> LDFQALEETTEYDGGYTRDSVLIREFWEIVHSFTDEQKRLFLQFTTGTDRAPVGGLGKLKMIIAKNGPDTERLPTSHTCFNVLLLPEYSSKEKLKERLLKAITYA

The HECT‐type ubiquitin ligase E6AP (UBE3A) is critically involved in several neurodevelopmental disorders and human papilloma virus‐induced cervical tumorigenesis; the structural mechanisms underlying the activity of this crucial ligase, however, are incompletely understood. E3s of the HECT (homologous to E6AP C‐terminus)‐subfamily share a C‐terminal catalytic domain that is comprised of two lobes—a ~30 kDa N‐lobe and a ~14 kDa C‐lobe—tethered by a flexible linker. Both lobes cooperate with each other in mediating sequential macromolecular interactions during ubiquitin transfer; in addition, the C‐lobe contains a catalytic cysteine that forms a thioester with the C‐terminus of ubiquitin in an intermediate step of catalysis. The founding member of the HECT E3 family, E6AP (UBE3A), has key roles in human diseases: its activity is hijacked by the E6 protein from high‐risk human papilloma viruses to promote the proteasomal degradation of the tumor suppressor p53, thereby driving cervical tumorigenesis; genetic up‐regulation of E6AP has been linked to autism spectrum disorders; and the deletion or down‐regulation of this ligase in the brain causes Angelman's syndrome.

We determined a crystal structure of the C‐lobe of E6AP at 1.3 Å resolution. The structure reveals a dimeric arrangement, in which the C‐terminal α‐helix (H14) and adjacent β‐strand (S10) of two symmetry‐related molecules have undergone three‐dimensional domain swapping. Interestingly, the hinge region that mediates the domain swap coincides with the active‐site region (Thr819, Cys820, Phe821, and Asn822) and adopts two conformations. As a consequence, the catalytic cysteine (Cys820) residues of the two subunits are either in immediate proximity or at a sulfur–sulfur distance of 4.7 Å, which we interpret as a mixture of disulfide‐bonded and reduced states. We speculate that these alternative oxidation states originate from radiation‐induced, partial cleavage of an intermolecular disulfide bond formed during the crystallization process. We and others have previously reported that the C‐lobe and the HECT domain of E6AP are monomeric in solution, consistent with cell‐based studies on the full‐length ligase. Either way, we posit that the observed domain swapping specifically occurs in the context of the isolated C‐lobe and is unlikely to happen in the presence of the N‐lobe. As for E6AP, the hinge region in HERC6 comprises the active site, yet the swapped region is slightly offset and the subunits are tilted by ~40° with respect to the E6AP C‐lobe dimer, thus positioning the catalytic cysteine residues of the two subunits at a distance of 11 Å. At the same time, the structural reorganization may indicate inherent conformational strain in the hinge region within the monomeric fold. In line with this notion, the hinge region is the shortest among the loops connecting individual β‐strands of the C‐lobe and may thus resemble a loaded spring that releases conformational tension upon swapping.> SMEKNEKEMEEEAEMKAVATSPSGRFLKFDIELGRGAFKTVYKGLDTETWVEVAWCELQDRKLTKAEQQRFKEEAEMLKGLQHPNIVRFYDSWESILKGKKCIVLVTELMTSGTLKTYLKRFKVMKPKVLRSWCRQILKGLQFLHTRTPPIIHRDLKCDNIFITGPTGSVKIGDLGLATLMRTSFAK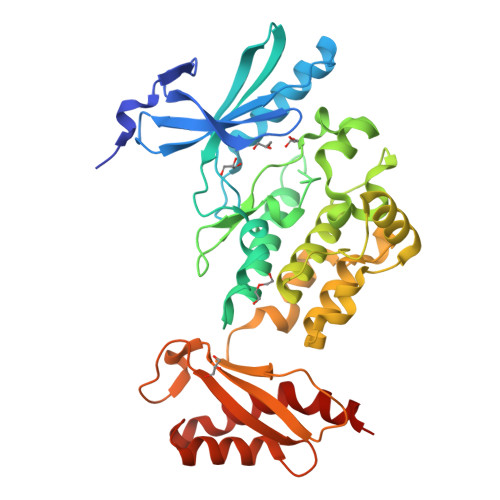SVIGTPEFMAPEMYEEHYDESVDVYAFGMCMLEMATSEYPYSECQNAAQIYRKVTSGIKPASFNKVTDPEVKEIIEGCIRQNKSERLSIRDLLNHAFFAEDTGLRVELAEEDDCSNSSLALRLWVEDPKKLKGKHKDNEAIEFSFNLETDTPEEVAYEMVKSGFFHESDSKAVAKSIRDRVTPIKKTREKKPA> MLRRSAVRYLKARPKTVNIEPGSNRFLDPNVEAKAKDIFAVPEFPNKAVLHNWRFFIKAGKAATGPPVGQEFSKLGLKAMDFAKAFNDRTKPHFKDDIELIVRIQVYFDKSYIFRIEPPPTAWFLLRAIRKKRGETGPVVLRGNYCAYLTLEMCYEIAKMKQMSWGKVEYPPIEVRVRRVVGQARRMGIAIIGIDTVHSSPVKGMTEKQYLEESEKHRKVHMIQYEALKAKELESAPLIERLHRPNMAPLTNTQLEEGLKDANLLNALWKSSHPKSLFTQDTRDR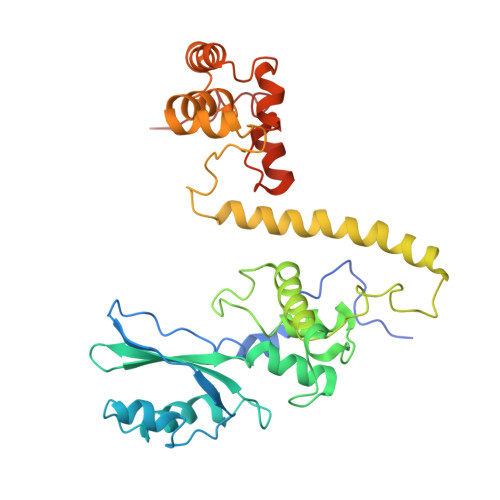EMARRYLNTRGWFKEMTPEEMRVVFLNYRLPKQEDHQRQLNMTNGQAQSQAYWSRDAASPQ> MKRNYILGLDIGITSVGYGIIDYETRDVIDAGVRLFKEANVENNEGRRSKRGARRLKRRRRHRIQRVKKLLFDYNLLTDHSELS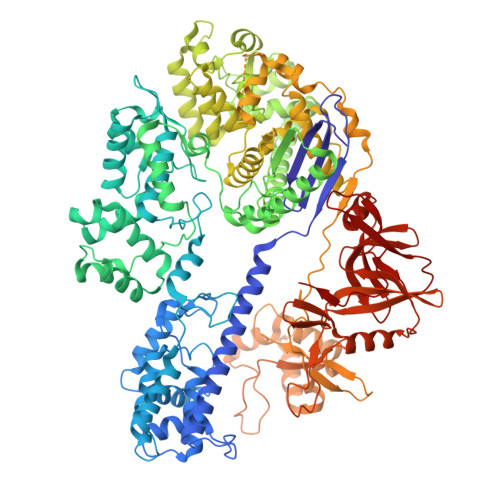GINPYEARVKGLSQKLSEEEFSAALLHLAKRRGVHNVNEVEEDTGNELSTKEQISRNSKALEEKYVAELQLERLKKDGEVRGSINRFKTSDYVKEAKQLLKVQKAYHQLDQSFIDTYIDLLETRRTYYEGPGEGSPFGWKDIKEWYEMLMGHCTYFPEELRSVKYAYNADLYNALNDLNNLVITRDENEKLEYYEKFQIIENVFKQKKKPTLKQIAKEILVNEEDIKGYRVTSTGKPEFTNLKVYHDIKDITARKEIIENAELLDQIAKILTIYQSSEDIQEELTNLNSELTQEEIEQISNLKGYTGTHNLSLKAINLILDELWHTNDNQIAIFNRLKLVPKKVDLSQQKEIPTTLVDDFILSPVVKRSFIQSIKVINAIIKKYGLPNDIIIELAREKNSKDAQKMINEMQKRNRQTNERIEEIIRTTGKENAKYLIEKIKLHDMQEGKCLYSLEAIPLEDLLNNPFNYEVDHIIPRSVSFDNSFNNKVLVKQEENSKKGNRTPFQYLSSSDSKISYETFKKHILNLAKGKGRISKTKKEYLLEERDINRFSVQKDFINRNLVDTRYATRGLMNLLRSYFRVNNLDVKVKSINGGFTSFLRRKWKFKKERNKGYKHHAEDALIIANADFIFKEWKKLDKAKKVMENQMFEEKQAESMPEIETEQEYKEIFITPHQIKHIKDFKDYKYSHRVDKKPNRELINDTLYSTRKDDKGNTLIVNNLNGLYDKDNDKLKKLINKSPEKLLMYHHDPQTYQKLKLIMEQYGDEKNPLYKYYEETGNYLTKYSKKDNGPVIKKIKYYGNKLNAHLDITDDYPNSRNKVVKLSLKPYRFDVYLDNGVYKFVTVKNLDVIKKENYYEVNSKCYEEAKKLKKISNQAEFIASFYNNDLIKINGELYRVIGVNNDLLNRIEVNMIDITYREYLENMNDKRPPRIIKTIASKTQSIKKYSTDILGNLYEVKSKKHPQIIKKG>[4x]MSDEMKKVMEALKKAVELAKKNNDDEVAREIERAAKEIVEALRENNSDEMAKVMLALAKAVLLAAKNNDDEVAREIAR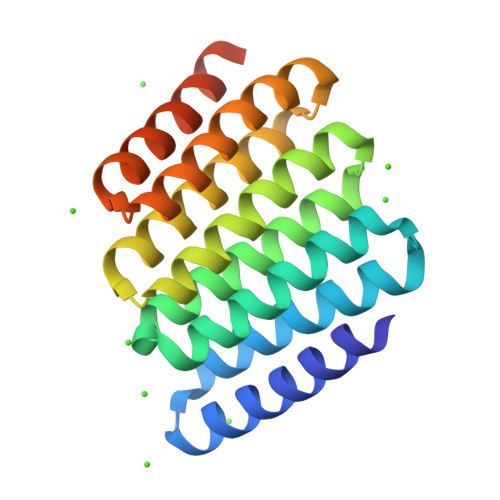AAAEIVEALRENNSDEMAKVMLALAKAVLLAAKNNDDEVAREIARAAAEIVEALRENNSDEMAKKMLELAKRVLDAAKNNDDETAREIARQAAEEVEADRENNSWLEHHHHHH Kinetochores, multisubunit protein assemblies, connect chromosomes to spindle microtubules to promote chromosome segregation. The 10-subunit KMN assembly (comprising KNL1, MIS12, and NDC80 complexes, designated KNL1C, MIS12C, and NDC80C) binds microtubules and regulates mitotic checkpoint function through NDC80C and KNL1C, respectively. The 10-subunit KMN assembly consists of three complexes, the 4-subunit MIS12 complex (MIS12C), the 2-subunit KNL1 complex (KNL1C), and the 4-subunit NDC80 complex (NDC80C) (Bharadwaj et al., 2004, Cheeseman et al., 2004, De Wulf et al., 2003, Desai et al., 2003, Kline et al., 2006, McCleland et al., 2003, Nekrasov et al., 2003, Obuse et al., 2004, Pinsky et al., 2003, Westermann et al., 2003, Wigge and Kilmartin, 2001). Human MIS12C (also known as MIND complex or Mtw1 complex in Saccharomyces cerevisiae) contains the MIS12, PMF1, NSL1, and DSN1 subunits (synonyms are reported in Table S1A). Finally, MIS12C is a binding hub that connects the other two KMN complexes to CCAN through an interaction with CENP-C (Gascoigne et al., 2011, Hori et al., 2013, Hornung et al., 2011, Hornung et al., 2014, Liu et al., 2016, Maskell et al., 2010, Petrovic et al., 2010, Przewloka et al., 2011, Screpanti et al., 2011).

From the results of limited proteolysis experiments (Petrovic et al., 2014), we engineered a deletion construct of the MIS12C in which three of the four subunits carried N- or C-terminal deletions. The resulting construct, referred to as MIS12CNano, did not crystallize, but addition of residues 1–71 of human CENP-C (CENP-C1–71), coupled with in situ proteolysis (Dong et al., 2007; STAR Methods), led to crystals. We collected X-ray diffraction data to minimum Bragg spacing of 3.5 Å from a native crystal and obtained initial phases from a tantalum bromide (Ta6Br122+) derivative in a different crystal form. The MIS12C is an extended rod, with a long axis of ∼200 Å (1 Å = 0.1 nm), in line with the previous low-resolution EM analyses. The four MIS12C subunits have similar topologies and span the entire length of the complex in the same orientation, so that all N and C termini cluster at opposite ends. The MIS12C subunits form two distinct subcomplexes, MIS12:PMF1 and DSN1:NSL1. The sturdy arrangement of helices in Head1 and in the helical connector of DSN1:NSL1 provides a composite binding site for CENP-C. The main chain of CENP-C resembles a “horseshoe. Its first visible segment (residues 6–22) is extended and binds in a shallow groove between the α1 and α2 helices of MIS12 in Head1. The CENP-C main chain then takes a turn (at Phe17CENP-C and Cys18CENP-C) to move away from the stalk through an extended and poorly conserved segment for which there is weak electron density. The CENP-C chain bends again to complete its “U-turn” around residues 28–30, emerging in helical conformation (residues 32–44, Figure 2C; a more detailed description of the interaction is in the legend of Figures S3A and S3B).

> MSVDPMTYEAQFFGFTPQTCMLRIYIAFQDYLFEVMQAVEQVILKKLDGIPDCDISPVQIRKCTEKFLCFMKGHFDNLFSKMEQLFLQLILRIPSNILLPEDKCKETPYSEEDFQHLQKEIEQLQEKYKTELCTKQALLAELEEQKIVQAKLKQTLTFFDELHNVGRDHGTSDFRESLVSLVQNSRKLQNIRDNVEKESKRLKIS;> MTISRVKLLDTMVDTFLQKLVAAGSYQRFTDCYKCFYQLQPAMTQQIYDKFIAQLQTSIREEISDIKEEGNLEAVLNALDKIVEEGKVRKEPAWRPSGIPEKDLHSVMAPYFLQQRDTLRRHVQKQEAENQQLADAVLAGRRQVEELQLQVQAQQQAWQALHREQRELVAVLREPE;> MSHQERLQSKSLHLSPQEQSASYQDRRQSWRRASMKETNRRKSLHPIHQGITELSRSISVDLAESKRLGCLLLSSFQFSIQKLEPFLRDTKGFSLESFRAKASSLSEELKHFADGLETDGTLQKCFEDSNGKASDFSLEASVAEMKEYITKFSLERQTWDQLLLHYQQEAKEILSRGSTEAKITEVKVEPMTYLGSSQNEVLNTKPDYQKILQNQSKVFDCMELVMDELQGSVKQLQAFMDESTQCFQKVSVQLGKRSMQQLDPSPARKLLKLQLQNPPAIHGSGSGSCQHHHHHH;> MAGSPELVVLDPPWDKELAAGTESQALVSATPREDFRVRCTSKRAVTEMLQLCGRFVQKLGDALPEEIREPALRDAQWTFESAVQENISINGQAWQEASDNCFMDSDIKVLEDQFDEIIVDIATKRKQYPRKILECVIKTIKAKQEILKQYHPVVHPLDLKYDPDPAPHMENLKCRGETVAKEISEAMKSLPALIEQGEGFSQVLR;> GPLGSMAASGLDHLKNGYRRRFCRPSRARDINTEQGQNVLEILQDCFEEKSLANDFSTNSTKSVPNSTRKIKDTCI>MTSTTTTTETLQEAVPFVAPPSPPEDVNNKELPEKPYYDVEFNYRLDPRDGGDEVIWGGTVGLMRRKYETRTVRINNERGNEHNFNLDTHGFAWVKHKTSVTEFADYLAIRQGPYYGEVAEMLKRVTGATKVHVIGHLHRSLNYNDTTEEEKNAPDMTMTKGQTPGRFVHVDQSYQGAVRRLYLDLPQEEARRLEKTRWAIINVWRPVRKVTNEPLAVCDARSVREDELFNTLHLVPMRWPDAAPQENQMWAVAPPKTPTQHKWHYVSGMTEDEALLIKMFDSKKDGTARRVPHSSFPTPDDFGEPRASTETRCF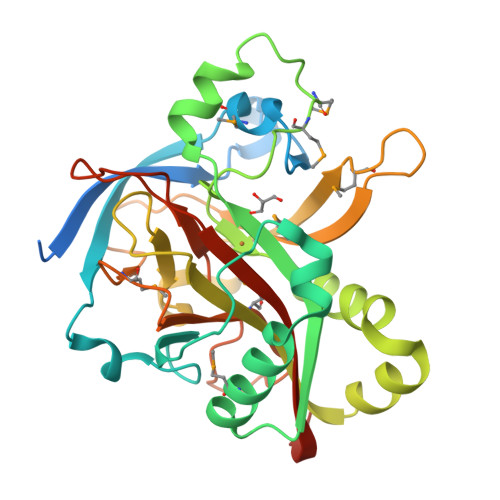VFWEDQEAEALEHHHHHH[2x]> MGDLPGIVRLSIALRIQPNDGPVFF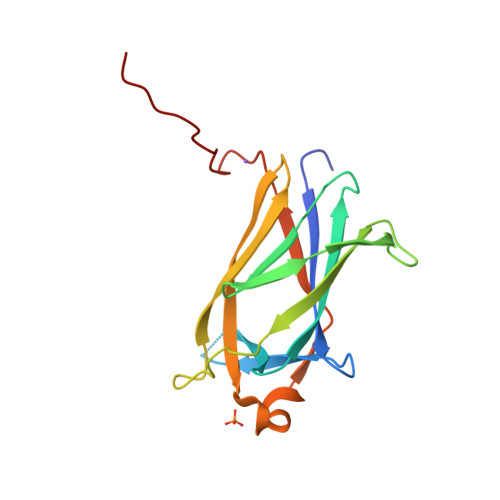KVDGQRFGQNRTIKLLTGSSYKVEVKIKPTTLQVENISIGGVLVPLELKCKEPDGERVVYTGIYDTEGVAPTKSGERQPIQITMPFTDIGTFETVWQVKFYNYHKRDHCQWGSPFSVIEYECKPNETRSLMWVNKESFL>VSKLINNGLLLVGQGAYQDLASPQQASVEQYNIIRFLGGAAPYIQNKGFGISTDIPDQCTLEQVQLFSRHGERYPSTGSGKKYKAVYEKLMSYNGTFKGELAFLNDDYEYFVPDSVYLEKETSPKNSDSIYAGTTDAMKHGIAFRTKYGELFDTNDTLPVFTSNSGRVYQTSQYFARGFMGDDFSNDTVKTNIISEDADMGANSLTPRDGCFNYNENANTAIVDEYTTEYLTKALNRFKASNPGLNITEDDVSNLFGYCAYELNVKGASP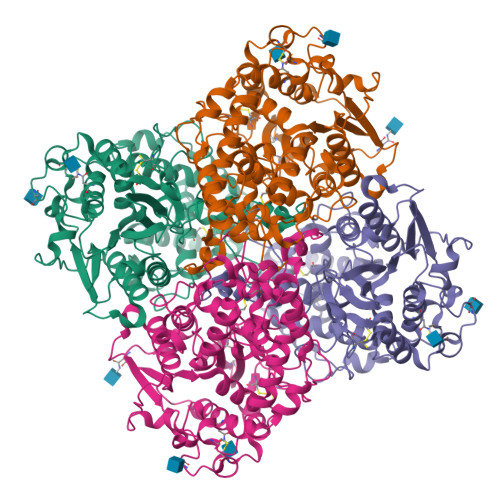MCDIFTNEEFIQYSYSVDLDDYYSNSAGNNMTRVIGSTLLNASLELLNHDKNENKIWLSFTHDTDIEIFHSAIGILIPDEDLPVDYTPFPSPYSHVGITPQGARTIIEKYACGNESYVRYVINDAVIPIKKCSSGPGFSCNLNDYNDYVAERVAGTNYVEQCGNNNASAVTFYWDYETTNYTASLINS[2x]> GPLGSMSLQEKLLTYYRNRAAIPAGEQARAKQAAVDICAELRSFLRAKLPDMPLRDMYLSGSLYDDLQVVTADHIQLIVPLVLEQNLWSCIPGEDTIMNVPGFFLVRRENPEYFPRGSSYWDRCVVGGYLSPKTVADTFEKVVAGSINWPAIGSLLDYVIRPAPPPEALTLEVQYERDKHLFIDFLPSVTLGDTVLVAKPHRLAQYDNLWRLSLRPAETARLRALDQADSGCRSLCLKILKAICKSTPALGHLTASQLTNVILHLAQEEADWSPDMLADRFLQALRGLISYLEAGVLPSALNPKVNLFAELTPEEIDELGYTLYCSLSEPEVLLQT

MiD51 and MiD49 are anchored in the mitochondrial outer membrane via their N-terminal ends, and most of the protein is exposed to the cytosol. MiD51 and MiD49 specifically interact with and recruit Drp1 to mitochondria and then facilitate Drp1-directed mitochondrial fission. Crystal structures of the cytosolic domains of MiD49 and MiD51 were reported and indicate that these proteins possess nucleotidyltransferase (NTase) folds and belong to the NTase family. MiD51 does bind adenosine diphosphate (ADP) as a cofactor, but MiD49 lacks this capacity.

To understand how MiD51 interacts with Drp1 during mitochondrial fission, we performed crystal structure studies and solved two types of MiD51 crystal structures under apo conditions. Type I contains the cytosolic domain MiD51129-463, and the crystal space group is P41212 with one molecule per asymmetric unit. The overall structure consists of a central β-strand region flanked by two α-helical regions and looks similar to NTPase family crystal structures published by two groups. The Type I and Type II crystal structures are almost identical, with a RMSD (root mean square deviation) variation of 1.14 Å for 329 aligned Cα atoms. By comparison, we found that all of the released crystal structures of MiD51 from PDB, which include different nucleotide forms (Apo, ADP or GDP), lack distinct conformational changes when compared to the Type I and Type II crystal structures, with RMSD variations ranging from 0.97 to 1.88 Å. And the ADP/GDP binding sites are almost identical, which implies the structural rigidity of MiD51. It was reported that MiD51 can form dimers primarily based on the crystal packing of MiD51, but we did not observe such packing in our two crystal types. DBS1, containing R234, Y240, F241 and R243, is located on an exposed loop of the N domain. We define this area as DBS2 (Drp1 Binding Site Two), which is located on α12 and α13 in the C domain and forms a surface for Drp1 binding. We also determined that MiD51 forms dimers through an interface close to residue C452 located in the C terminal region, although the majority of MiD51 protein exists as monomer.> 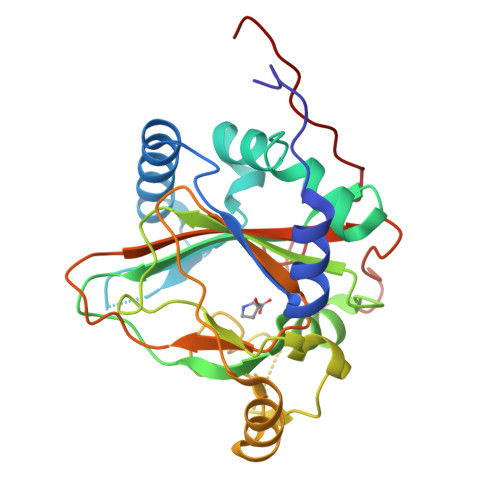QIMEPHDTLSPAQVDEYRKNGFLVQEHVFDEEEIELLRAEAAQEFASGGERVTVEQNTGIVRGVHGCHLYSEVFGRLVRSPRLLPIARQLLRDDVYVHQFKINAKRAFKGEVWEWHQDYTFWHHEDGMPAPRALSAAIFLDEVTEFNGPLTFVPGGHGSGMIDADVKGEGWANTLTASLKYSLDVETMRGLIERNGMVAPKGPRGSVLWFDANIPHSSVPNISPFDRGLVLITYNSVENKTDVTRGTRPEWLAARDFTPLTALQATSF>XDYLRELLKLELQLIKQYREALEYVKLPVLAKILEDEEKHIEWLETILGX[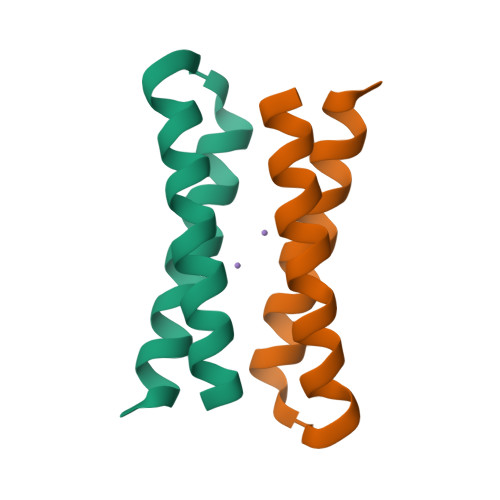4x]Finally, the CDPME2P is converted into MEcDP with concomitant release of CMP by MEcDP synthase (IspF). In this study, crystal structures of BsIspF in native and complexed with CMP have been determinated both at 1.99-Å resolutions. The monomer displays an α/β fold constructed with a four-strand β-sheet of β1, β2, β3, and β4, with β2 antiparallel to the others on one side, and a three-helix bundle of α1 to α3 on the other. In BsIspF trimer, the four-strand β-sheet of each subunit lay roughly parallel to the threefold NCS axis, forming a compact bell-shaped trimer of approximately 45 × 60 Å in the axial and equatorial dimensions, respectively.

CMP acts as the leaving group to give the cyclic diphosphate reaction product MEcDP. In the BsIspF/CMP complex, only four CMP moieties can be modeled in the six active pockets of the two trimers in the asymmetric unit with the occupancy higher than 0.7, one trimer fully loads CMP substrates, and the other captures only one. Although the two trimers in the asymmetric unit display extremely structural similarity (r.m.s.d: 0.20 Å), the B-factors of the active pocket in the two trimers are quite different, which may be the possible cause for this asymmetric binding. The CMP moieties reveal similar interactions with the protein. The cytidine group of CMP interacts with the residues Ala101, Pro104, Met106, and Leu107 through main-chain atoms, and the ribose hydroxyl groups form hydrogen bonds with the carboxylate of Asp57 and the amide of Gly59 from the adjacent subunits. Residues Thr133 and Thr134 hydrogen bond to the α-phosphate of CMP, waters act as a bridge between the α-phosphate and the magnesium ion. All these residues are highly conserved in the IspF protein. And, the overlay of each chain between the native and BsIspF/CMP complex reveal r.m.s.d values ranging from 0.12 to 0.24 Å. Moreover, structural comparisons show that only a small Cα r.m.s.d differences (~0.1 Å) occur in this region between BsIspF and BsIspF/CMP complex. In both native and CMP bonded structures of BsIspF, magnesium ions were refined in the active site, with the ingredient of magnesium ions used in the crystallization cocktail.

>[6x]MFRIGQGFDVHQLVEGRPLIIGGIEIPYEKGLLGHSDADVLLHTVADACLGAVGEGDIGKHFPDTDPEFKDADSFKLLQHVWGIVKQKGYVLGNIDCTIIAQKPKMLPYIEDMRKRIAEGLEADVSQVNVKATTTEKLGFTGRAEGIAAQATVLIQKG>[2x]MVLYFIGLGLYDERDITVKGLEIAMKCDYVFAEFYTSLMAGTTLGRIQKLIGKEIRVLSREDVELNFENIVLPLAKENDVAFLTPGDPLVATTHAELRIRAKRAGVESYVIHAPSIYS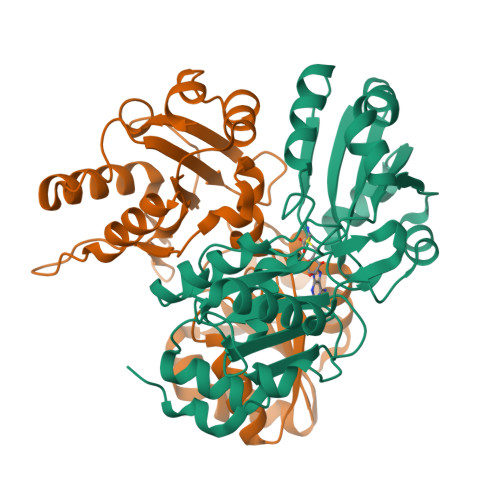AVGITGLHIYKFGKSATVAYPEGNWFPTSYYDVIKENAERGLHTLLFLDIKAEKRMYMTANEAMELLLKVEDMKKGGVFTDDTLVVVLARAGSLNPTIRAGYVKDLIREDFGDPPHILIVPGKLHIVEAEYLVEIAGAPREILRVNV> EGGVAMPG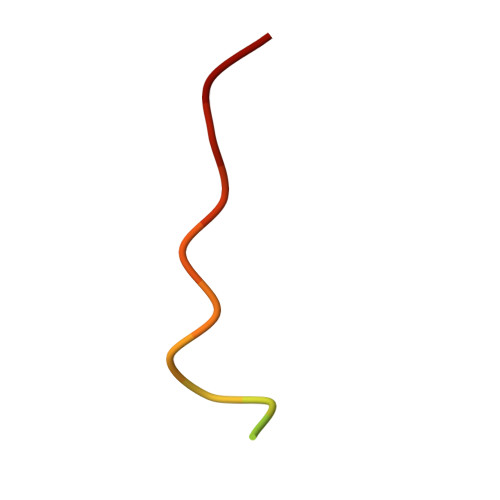AEDDVVTPGC> AATYAQTLQNIPETNVTTLDNGLRVASEESSQPTCTVGVWIGAGSRYENEKNNGAGYFVEHLAFKGTKKRPCAAFEKEVESMGAHFNGYTSREQTAFYIKALSKDMPKVVELLADVVQNCALEESQIEKERGVILQELKEMDNDMTNVTFDYLHATAFQGTALARTVEGTTENIKHLTRADLASYIDTHFKAPRMVLAAAGGISHKELVDAARQHFSGVSFTYKEDAVPILPRCRFTGSEIRARDDALPVAHVALAVEGPGWADPDNVVLHVANAIIGRYDRTFGGGKHLSSRLAALAVEHKLCHSFQTFNTSYSDTGLFGFHFVADPLSIDDMMFC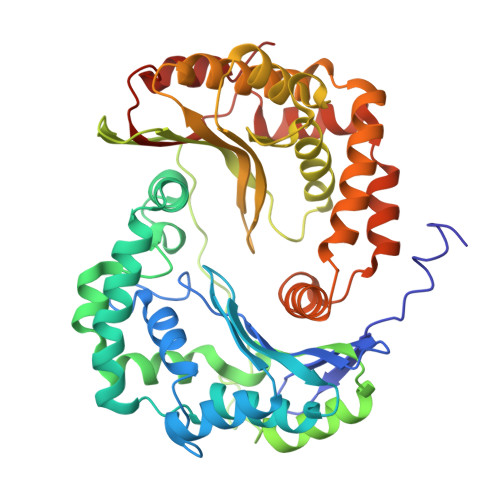AQGEWMRLCTSTTESEVKRAKNHLRSAMVAQLDGTTPVCETIGSHLLNYGRRISLEEWDSRISAVDARMVRDVCSKYIYDKCPALAAVGPIEQLLDYNRIRSGMYWIRF methyl 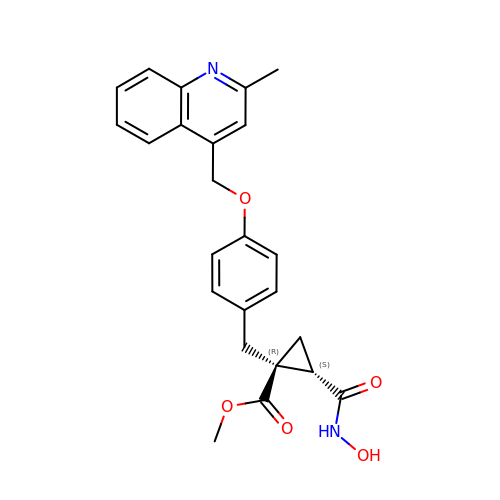(1R,2S)-2-(hydroxycarbamoyl)-1-{4-[(2-methylquinolin-4-yl)methoxy]benzyl}cyclopropanecarboxylate | C24 H24 N2 O5 | HJWMYFBKJRVWJY-YKSBVNFPSA-N> GPGADGWLELESDPGLFTLLLKDFGCHDVQVEEVYDLQKPIESPYGFIFLFRWIEERRARRKIVETTAEIFVKDEEAISSIFFAQQVVPNSCATHALLSVLLNCNENNLQLGDTLSRLKTHTKGMSPENKGLAIGNTPELACAHNSHAMPQARRRLERTGAGVSSCRFTGEAFHFVSFVPINGQLFELDGLK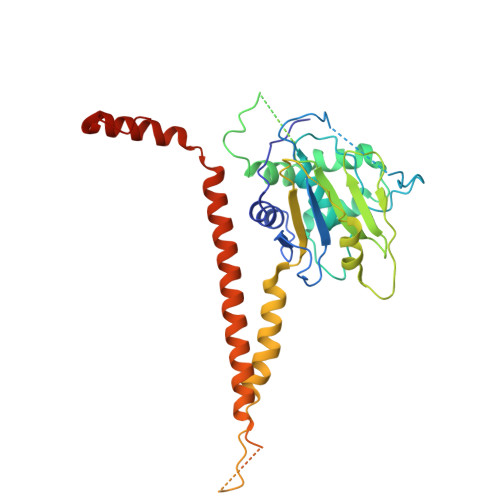PYPMNHGGWEDSEDWTDKFRRVMAERLGIATGEQDIRFNLMAVVPDRRIAITHKLKMLRTNQAIVSGTLQKLLKADEQGESGNGDSQRPDTPTTLLEPSAFTARDLQSLLKNLDTEIAINEQHLADENDRRHMFKVDASRRTHNYDKFICTFLSMLAHQGVLGELVSQHLLPS>TDTTLPPDDSLDRIEPVDIEQEMQRSYIDYAMSVIVGRALPEVRDGLKPVHRRVLYAMFDSGFRPDRSHAKSARSVAETMGNYHPHGDASIYDSLVRMAQPWSLRYPLVDGQGNFGSPGNDPPAAMRYTEARLTPLAMEMLREIDEETVDFIPNYDGRVQEPTVLPSRFPNLLANGSGGIAVGMATNIPPHNLRELADAVFWALENHDADEEETLAAVMGRVKGPDFPTAGLIVGSQGTADAYKTGRGSIRMRGVVEVEEDSRGRTSLVITELPYQVNHDNFITSIAEQVRDGKLAGISNIEDQSSDRVGLRIVIEIKRDAVAKVVINNLYKHTQLQTSFGANMLAIVDGVPRTLRLDQLIRYYVDHQLDVIVRRTTYRLRKANERAHILRGLVKALDALDEVIALIRASETVDIARAGLIELLDIDEIQAQAILDMQLRRLAALERQRIIDDLAKIEAEIADLEDILAKPERQRGIVRD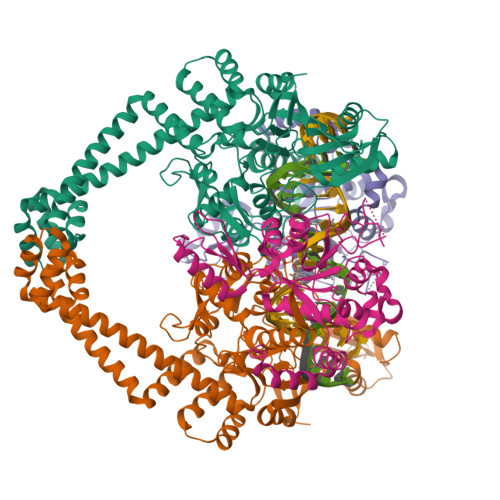ELAEIVDRHGDDRRTRIIAIGSG[2x];>SNALVRRKSATDIGGLPGKLADCRSTDPRKSELYVVEGDSAGGSAKSGRDSMFQAILPLRGKIINVEKARIDRVLKNTEVQAIITALGTGIHDEFDIGKLRYHKIVLMADADVDGQHISTLLLTLLFRFMRPLIENGHVFLAQPPLYKLKWQRSDPEFAYSDRERDGLLEAGLKAGKKINKEDGIQRYKGLGEMDAKELWETTMDPSVRVLRQVTLDDAAAADELFSILMGEDVDARRSFITRNAKDVRFLDV[2x]TAZOBACTAM | C10 H12 N4 O5 S | 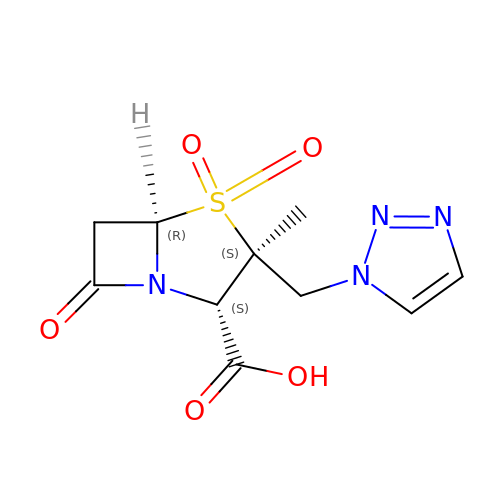LPQZKKCYTLCDGQ-WEDXCCLWSA-N>[2x]MKGIIFNVLEDMVVAQCGMSVWNELLEKHAPKDRVYVSAKSYAESELFSIVQDVAQRLNMPIQDVVKAFGQFLFNGLASRHTDVVDKFDDFTSL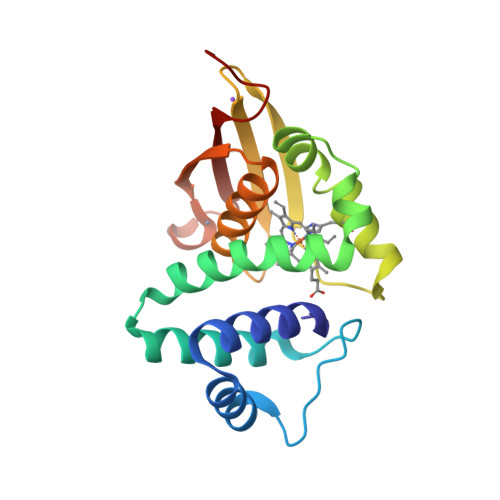VMGIHDVIHLEVNKLYHEPSLPHINGQLLPNNQIALRYSSPRRLCFCAEGLLFGAAQHFAAAIQISHDTCMHTGADHCMLIIELQNDENLYFQ>GHSGYRPNLLARNLSAKSTQTLGLVVTNTLYHGIYFSELLFHAARMAEEKGRQLLLADGKHSAEEERQAIQYLLDLRCDAIMIYPRFLSVDEIDDIIDAHSQPIMVLNRRLRKNSSHSVWCDHKQTSFNAVAELINAGHQEIAFLTGSMDSPTSIERLAGYKDALAQHGIALNEKLIANGKWTPASGAEGVEMLLERGAKFSALVASNDDMAIGAMKALHERGVAVPEQVSVIGFDDIAIAPYTVPALSSVKIPVTEMIQEIIGRLIFMLDGGDFSPPKTFSGKLIRRDSLI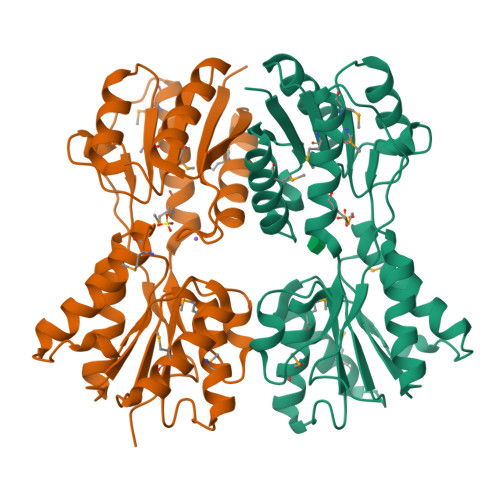APSR[2x]> YNTVSFNLGEAYEYPTFIQDLRNELAKGTPVCQLPVTLQTIADDKRFVLVDITTTSKKTVKVAIDVTDVYVVGYQDKWDGKDRAVFLDKVPTVATSKLFPGVTNRVTLTFDGSYQKLVNAAKVDRKDLELGVYKLEFSIEAIHGKTINGQEIAKFFLIVIQMVSEAARFKYIETEVVDRGLYGSFKPNFKVLNLENNWGDISDAIHKSSPQCTT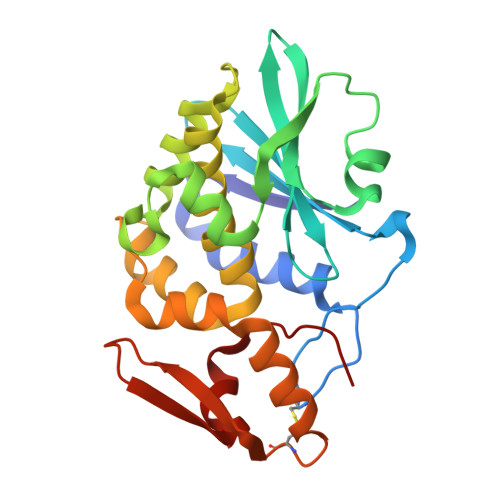INPALQLISPSNDPWVVNKVSQISPDMGILKFKS> GPAFEFAVAMMKRNSSTVKTEYGEFTMLGIYDRWAVLPRHAKPGPTILMNDQEVGVLDAKELVDKDGTNLELTLLKLNRNEKFRDIRGFLAKEEVEVNEAVLAINTSKFPNMYIPVGQVTEYGFLNLGGTPTKRMLMYNFPTRAGQCGGVLMSTGKVLGIHVGGNGHQGFSAALLKHYFN

Among them, we have the proteases encoded by the 3C region of the enteroviruses genome (3CPro, hereafter), such as Coxsackievirus B3 (CVB3), EV-D68, EV-A71 and Coxsackievirus A16. The fact that all these virally encoded proteases from coronaviruses and enteroviruses perform essential functions in the viral replication cycle by cleaving both viral and host targets, as well as the fact that there is no known human protease with a specificity for Gln at the cleavage site of the substrate, has pushed the scientific community towards the development of a commercially viable antiviral drug targeting both of these virus families. While this dimerization is essential for the catalytic activity of 3CLPro, the enteroviral 3Cpro functions as a monomer. The structure of CVB3-3Cpro adopts a chymotrypsin protein fold.

The crystal structure of CVB3 3CPro in complex with the GC-376 PROTAC precursor was solved at 1.9 Å resolution, which provided atomic details of the CVB3 3CPro–ligand interactions. The N-terminus starts with an α-helix of residues 1–14 and is followed by two topologically equivalent β-barrels comprising residues 15–77 and 100–173, which pack together to form a narrow groove for substrate binding. The catalytic triad of Cys147, His40 and Glu71 is located in the cleft between the two β-barrels. The most relevant feature is the binding mode of the ligand to the catalytic Cys147, which occurs via a covalent bond between C5 and the sulfur atom of Cys147. From a crystallographic point of view, this is supported by the fact that the bond length spontaneously refines to values around 1.8 Å, which is coherent with a C-S covalent bond. The protein atoms involved in direct hydrogen bond interactions with the ligand are, namely, the backbone oxygen of Thr142, one of the imidazole nitrogen atoms of His161, the backbone oxygen of Val162, the backbone nitrogen atom of Gly164 and the backbone nitrogen atom of Cys147. The only exception is the conformation of the phenyl ring of the benzyloxycarbonyl group, which is basically flipped by 90°. This effect is due to a different structural arrangement of the C-terminal segment of CVB3 3CPro with respect to that of SARS-CoV-2 3CLPro, which makes the substrate cavity of CVB3 3CPro more open. The larger available volume allows the phenyl ring to rotate in a position that is structurally more congested in the structure of SARS-CoV-2 3CLPro. Specifically, the GC-376 PROTAC showed 32 ± 3% inhibition at 100 μM, and the GC-376 PROTAC precursor showed an IC50 of 4.6 μM (pIC50 = 5.28 ± 0.07).> MAGNFSEIES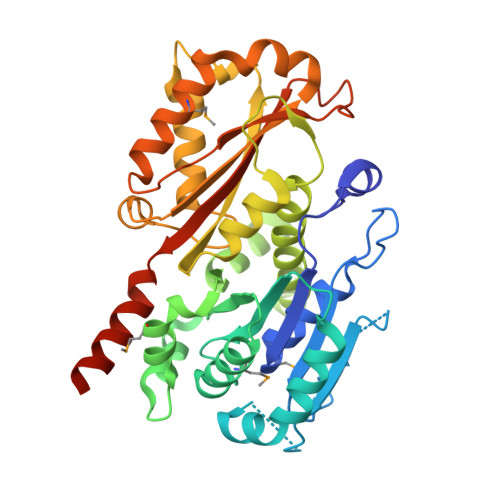QGNISLKFGFLGLGMGGCAIAAECANKETQIKNNKYPYRAILVNTNSQDFNKIEIKNTGNVRKIQLEGYEQGAARNPQVGEEAFVKHETKIFEAVKQEFEDRDFIWITCGLGGGTGTGALLKAIEMLYEHDYNFGLLLTLPRDAEALKVLENATSRIRSIAMNQEAFGSIVLIDNAKLYRKFEEENPSALANEYTSYSNKYIADALHEINLVTSSFTPFSDTHFDASEFAQVINTPGVLSLAKLELKSNQLDTENPLGYLTQLGNALEKGVLYDTEREELESAKKSALSIVTSPLRAGRLYNFSFLNQMENFLKERTPYVDERPIAPYVNKHTTKKEEDIVKFYSVVAGLPLPKRVSDIIDEITRIKEEREQANSKKSN> GAKPERGRFLHFHSVTFWVGNAKQAASFYCSKMGFEPLAYRGLETGSREVVSHVIKQGKIVFVLSSALNPWNKEMGDHLVKHGDGVKDIAFEVEDCDYIVQKARERGAKIMREPWVEQDKFGKVKFAVLQTYGDTTHTLVEKMNYIGQFLPGYEAPAFMDPLLPKLPKCSLEMIDHIVGNQPDQEMVSASEWYLKNLQFHRFWSVDDTQVHTEYSSLRSIVVANYEESIKMPINEPAPGKKKSQIQEYVDYNGGAGVQHIALKTEDIITAIRHLRERGLEFLSVPSTYYKQLREKLKTAKIKVKENIDALEELKILVDYDEKGYLLQIFTKPVQDRPTLFLEVIQRHNHQGFGAGNFNS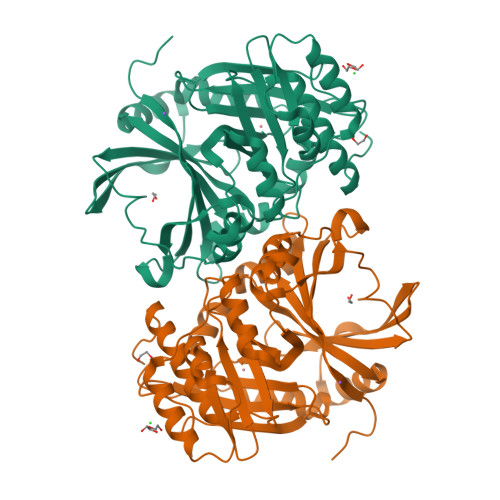LFKAFEEEQNLRGNLTNMETNGVVPGMAENLYFQ>MGSDKIHHHHHHMTNANGNLKKCPITISSYTLGTEVSFPKRVKVAAENGFDGIGLRAENYVDALAAGLTDEDMLRILDEHNMKVTEVEYITQWGTAEDRTAEQQKKEQTTFHMARLFGVKHINCGLLEKIPEEQIIVALGELCDRAEELIIGLEFMPYSGVADLQAAWRVAEACGRDNAQLICDTWHWARANQTAESIKNVPADRIVSIQLCDVHETPYKELREESLHDRLAPGEGYGDTVGFAKILKEHGVNPRVMGVEVIS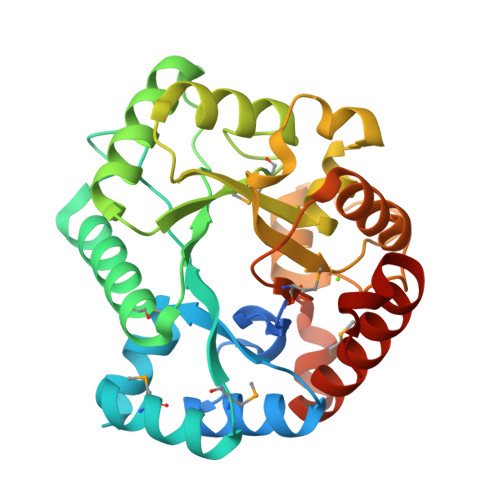DSMVATGLEYAALKVYNATKKVLDEAWPEISPR[2x]HEXAETHYLENE 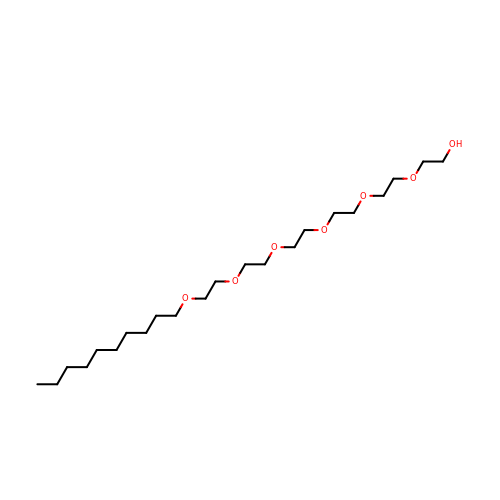GLYCOL MONODECYL ETHER | C22 H46 O7 | GLGQRQQFWLTGES-UHFFFAOYSA-N>AVIDIDAATKIMCSNAKAISLNEVEKNEIISKYREITAKKSERAELKEVEPIPLDWPSDLTLPPLPESTNDYVWAGKRKELDDYPRKQLIIDGLSIVIPTYNRAKILAITLACLCNQKTIYDYEVIVADDGSKENIEEIVREFESLLNIKYVRQKDYGYQLCAVRNLGLRAAKYNYVAILDCDMAPNPLWVQSYMELLAVDDNVALIGPRKYIDTSKHTYLDFLSQKSLINEIPEIITNNQVAGKVEQNKSVDWRIEHFKNTDNLRLCNTPFRFFSGGNVAFAKKWLFRAGWFDEEFTHWGGEDNEFGYRLYREGCYFRSVEGAMAYHQEPPGKENETDRAAGKNITVQLLQQKVPYFYRKKEKIESATLKRVPLVSIYIPAYNCSKYIVRCVESALNQTITDLEVCICDDGSTDDTLRILQEHYANHPRVRFISQKNKGIGSASNTAVRLCRGFYIGQLDSDDFLEPDAVELCLDEFRKDLSLACVYTTNRNIDREGNLISN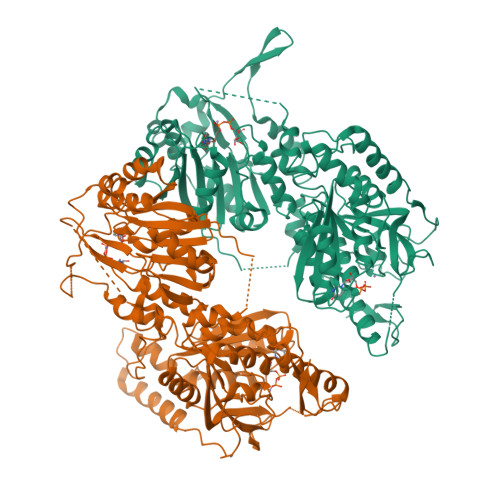GYNWPIYSREKLTSAMICHHFRMFTARAWNLTEGFNESISNAVDYDMYLKLSEVGPFKHINKICYNRVLHGENTSIKKLDIQKENHFKVVNESLSRLGIKKYKYSPLTNLNECRKYTWEKI[2x]>[2x]MVEKEEAGGGISEEEAAQYDRQIRLWGLEAQKRLRASRVLLVGLKGLGAEIAKNLILAGVKGLTMLDHEQVTPEDPGAQFLIRTGSVGRNRAEASLERAQNLNPMVDVKVDTEDIEKKPESFFTQFDAVCLTCCSRDVIVKVDQICHKNSIKFFTGDVFGYHGYTFANLGEHEFVEEKTKVAKVSQGVEDGPDTKRAKLDSSETTMVKKKVVFCPVKEALEVDWSSEKAKAALKRTTSDYFLLQVLLKFRTDKGRDPSSDTYEEDSELLLQIRNDVLDSLGISPDLLPEDFVRYCFSEMAPVC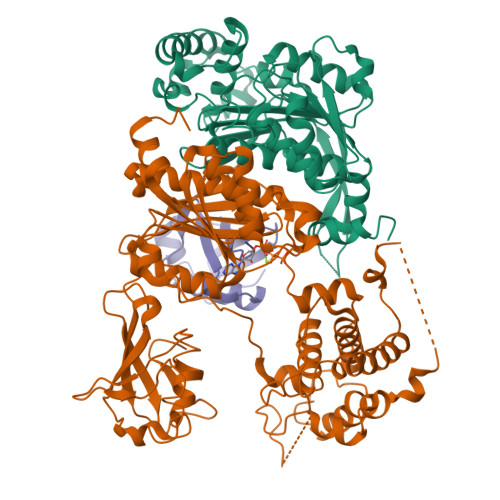AVVGGILAQEIVKALSQRDPPHNNFFFFDGMKGNGIVECLGPK;>[2x]MALSRGLPRELAEAVAGGRVLVVGAGGIGCELLKNLVLTGFSHIDLIDLDTIDVSNLNRQFLFQKKHVGRSKAQVAKESVLQFYPKANIVAYHDSIMNPDYNVEFFRQFILVMNALDNRAARNHVNRMCLAADVPLIESGTAGYLGQVTTIKKGVTECYECHPKPTQRTFPGATIRNTPSEPIHCIVWAKYLFNQLFGEEDADQEVSPDRADPEAAWEPTEAEARARASNEDGDIKRISTKEWAKSTGYDPVKLFTKLFKDDIRYLLTMDKLWRKRKPPVPLDWAEVQSQGEETNASDQQNEPQLGLKDQQVLDVKSYARLFSKSIETLRVHLAEKGDGAELIWDKDDPSAMDFVTSAANLRMHIFSMNMKSRFDIKSMAGNIIPAIATTNAVIAGLIVLEGLKILSGKIDQCRTIFLNKQPNPRKKLLVPCALDPPNPNCYVCASKPEVTVRLNVHKVTVLTLQDKIVKEKFAMVAPDVQIEDGKGTILISSEEGETEANNHKKLSEFGIRNGSRLQADDFLQDYTLLINILHSEDLGKDVEFEVVGDAPEKVGPKQAEDAAKSITNGSDDGAQPSTSTAQEQDDVLIVDSDEEDSSNNADVSEEERSRKRKLDEKENLSAKRSRIEQKEELDDVIALD;>[2x]MSDQEAKPSTEDLGDKKEGEYIKLKVIGQDSSEIHFKVKMTTHLKKLKESYCQRQGVPMNSLRFLFEGQRIADNHTPKELGMEEEDVIEVYQEQTGG> GPGHMPEYQAQGLAMYLQENGIDCPKCKFSYALARGGCMHFHCTQCRHQFCSGCYNAFYAKNKCPEPNCRVKKSL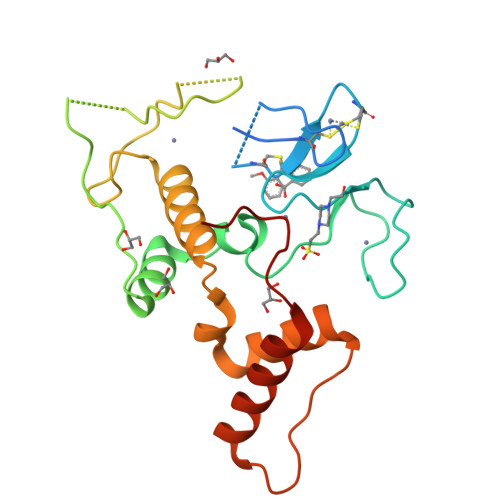HGHHPRDCLFYLRDWTALRLQKLLQDNNVMFNTEPPAGARAVPGGGCRVIEQKEVPNGLRDEACGKETPAGYAGLCQAHYKEYLVSLINAHSLDPATLYEVEELETATERYLHVRPQPLAGEDPPAYQARLLQKLTEEVPLGQSIPRRRK> XPPGPPGPPGPRGFPGPPGPP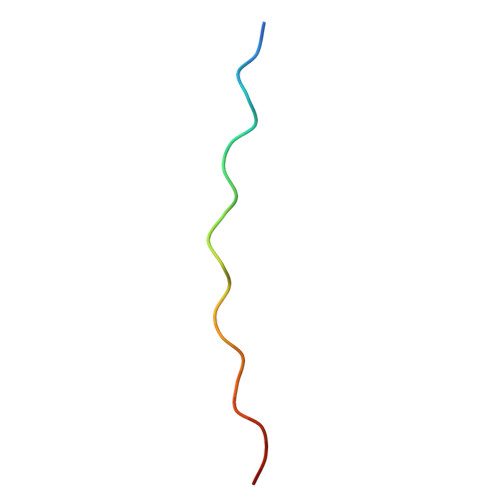G>GHKPEPTDEEWELIKTVTEAHVATNAQGSHWKQKRKFLPEDIGQAPIVNAPEGGKVDLEAFSHFTKIITPAITRVVDFAKKLPMFCELPCEDQIILLKGCCMEIMSLRAAVRYDPESETLTL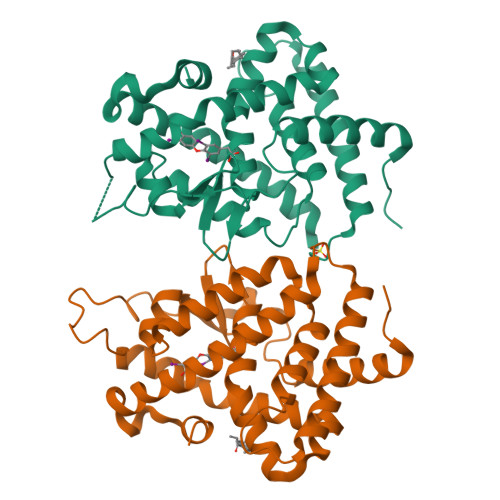NGEMAVTRGQLKNGGLGVVSDAIFRLGMSLSSFNLDDTEVALLQAVLLMSSDRPGLACVERIEKYQDSFLLAFEHYINYRKHHVTHFWPKLLMKVTDLRMIGACHASRFLHMKVECPTELFPPLFLEVFED[2x]>[2x]MRPSAPAISRQTLLDEPRPGSLTIGYEPSEEAQPTENPPRFSWLPDIDDGARYVLRISTDPGFTDKKTLVFEDLAWNFFTPDEALPDGHYHWCYALWDQKSATAHSNWSTVRSFEISEALPKTPLPGRSARHAAAQTSHPRLWLNSEQLSAFADAVAKDPNHCGWAEFYEKSVEPWLERPVMPEPQPYPNNTRVATLWRQMYIDCQEVIYAIRHLAIAGRVLGRDDLLDASRKWLLAVAAWDTKGATSRAYNDEAGFRVVVALAWGYDWLYDHLSEDERRTVRSVLLERTREVADHVIAHARIHVFPYDSHAVRSLSAVLTPACIALQGESDEAGEWLDYTVEFLATLYS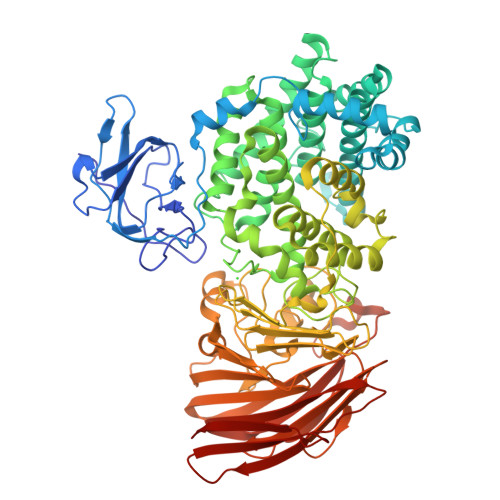PWAGTDGGWAEGPHYWMTGMAYLIEAANLIRSYIGYDLYQRPFFQNTGRFPLYTKAPGTRRANFGDDSTLGDLPGLKLGYNVRQFAGVTGNGHYQWYFDHIKADATGTEMAFYNYGWWDLNFDDLVYRHDYPQVEAVSPADLPALAVFDDIGWATIQKDMEDPDRHLQFVFKSSPYGSLSHSHGDQNAFVLYAHGEDLAIQSGYYVAFNSQMHLNWRRQTRSKNAVLIGGKGQYAEKDKALARRAAGRIVSVEEQPGHVRIVGDATAAYQVANPLVQKVLRETHFVNDSYFVIVDEVECSEPQELQWLCHTLGAPQTGRSSFRYNGRKAGFYGQFVYSSGGTPQISAVEGFPDIDPKEFEGLDIHHHVCATVPAATRHRLVTLLVPYSLKEPKRIFSFIDDQGFSTDIYFSDVDDERFKLSLPKQF>[2x]AGFKPAPPAGQLGAVIVDPYGNAPLTALVDLDSHVISDVKVTVHGKGEKGVEISYPVGQESLKTYDGVPIFGLYQKFANKVTVEWKENGKVMKDDYVVHTSAIVNNYMDNRSISDLQQTKVIKVAPGFEDRLYLVNTHTFTAQGSDLHWHGEKDKNAGILDAGPATGALPFDIAPFTFIVDTEGEYRWWLDQD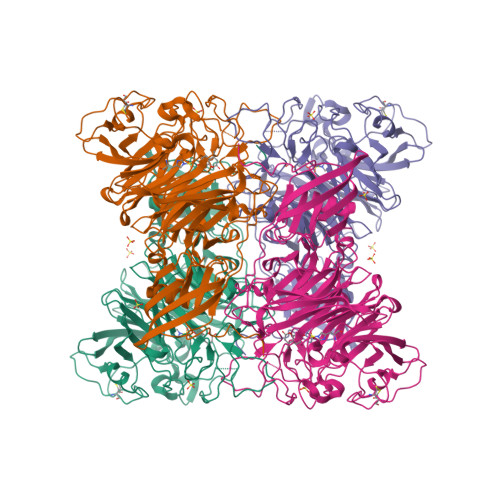TFYDGRDRDINKRGYLMGIRETPRGTFTAVQGQHWYEFDMMGQVLEDHKLPRGFADATHESIETPNGTVLLRVGKSNYRRDDGVHVTTIRDHILEVDKSGRVVDVWDLTKILDPKRDALLGALDAGAVCVNVDLAHAGQQAKLEPDTPFGDALGVGPGRNWAHVNSIAYDAKDDSIILSSRHQGVVKIGRDKQVKWILAPSKGWEKPLASKLLKPVDANGKPITCNENGLCENSDFDFTYTQHTAWISSKGTLTIFDNGDGRHLEQPALPTMKYSRFVEYKIDEKKGTVQQVWEYGKERGYDFYSPITSIIEYQADRNTMFGFGGSIHLFDVGQPTVGKLNEIDYKTKEVKVEIDVLSDKPNQTHYRALLVRPQQMFK>MRGSHHHHHHGSMDAQSAAKCLTAVRRHSPLVHSITNNVVTNFTANGLLALGASPVMAYAKEEVADMAKIAGALVLNIGTLSKESVEAMI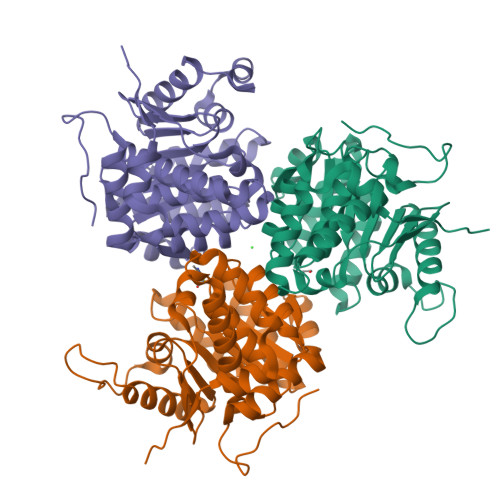IAGKSANEHGVPVILDPVGAGATPFRTESARDIIREVRLAAIRGNAAEIAHTVGVTDWLIKGVDAGEGGGDIIRLAQQAAQKLNTVIAITGEVDVIADTSHVYTLHNGHKLLTKVTGAGCLLTSVVGAFCAVEENPLFAAIAAISSYGVAAQLAAQQTADKGPGSFQIELLNKLSTVTEQDVQEWATIERVTVS[3x]> MTKDLNTLVSELPEIYQTIFGHPEWDGDAARDCNQRLDLITEQYDNLSRALGRPLNVLDLGCAQGFFSLSLASKGATIVGIDFQQENINVCRALAEENPDFAAEFRVGRIEEVIAALEEGEFDLAIGLSVFHHIVHLHGIDEVKRLLSRLADVTQAVILELAVKEEPLYWGVSQPDDPRELIEQCAFYRLIGEFDTHLSPVPRPMYLVSNHRVLINDFNQPFQHWQNQPYAGAGLAHKRSRRYFFGEDYVCKFFYYDMPHGILTAEESQRNKHELHNEIKFLTQPPAGFDAPAVLAHGENAQSGWLVMEKLPGRLLSDMLAAGEEIDREKILGSLLRSLAALEKKGFWHDDVRPWNVMVDARQHARLIDFGSIVTTPQDCSWPTNLVQSFFVFVNELFAENKSWNGFWRSAPVHPFNLPQPWS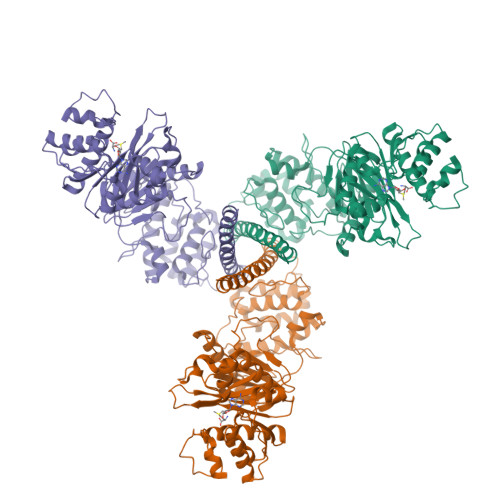NWLYAVWQEPVERWNFALLLALFEKKAKLPSAEQQRGATEQWIIAQETVLLELQSRVRNESAGSEALRGQIHTLEQQMAQLQ>LSFTLEEEDITGTWYVKAMVVDKDFPEDRRPRKVSPVKVTALGGGNLEATFTFMREDRCI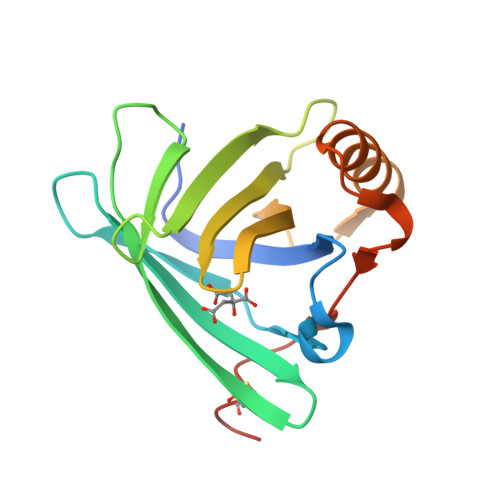QKKILMRKTEEPGKFSAYGGRKLIYLQELPGTDDYVFYSKDQRRGGLRYMGNLVGRNPNTNLEALEEFKKLVQHKGLSEEDIFMPLQTGSCVLEHHHHHHH[2x]>[2x]MDLTNKNVIFVAALGGI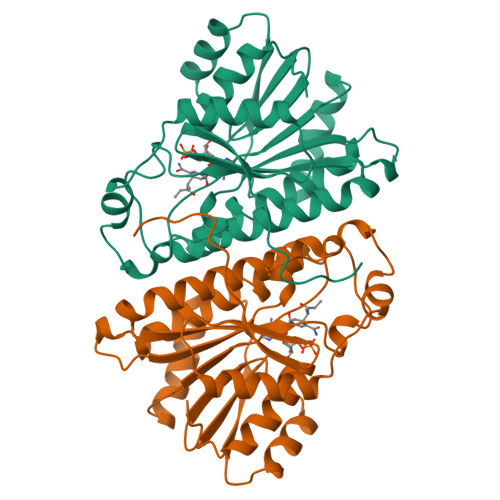GLDTSRELVKRNLKNFVILDRVENPTALAELKAINPKVNITFHTYDVTVPVAESKKLLKKIFDQLKTVDILINGAGILDDHQIERTIAINFTGLVNTTTAILDFWDKRKGGPGGIIANICSVTGFNAIHQVPVYSASKAAVVSFTNSLAKLAPITGVTAYSINPGITRTPLVHTFNSWLDVEPRVAELLLSHPTQTSEQCGQNFVKAIEANKNGAIWKLDLGTLEAIEWTKHWDSHI>SNAMKEPPMTKTVFHLGVTEADLNGATLAIIPGDPARVQKIAELMDNPVFLASHREYTVYRAELDGQSVVVCSTGIGGPSTSIAVEELAQLGVRTFLRVGTTGAIQPHVNVGDMIVTTGSVRLDGASLHFAPMEFPAVPDFDVATAMKAAAQESGATVHMGVTASSDTFYPGQERYDTFTGRVVRRFQGSMKEWQDMGVLNF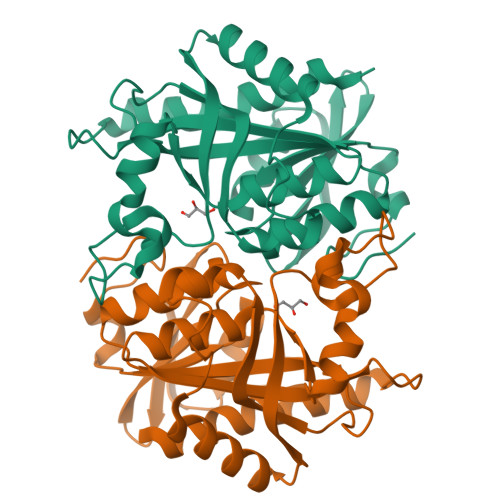EMESATLLTMCASSGLKAGCVAGVIINRTQKEIPDHATLKETEARSIKVVVEAARKMLK[2x]(2E,5R)-5-[3-(5-chloropyridin-3-yl)phenyl]-5-cyclopropyl-2-imino-3-methylimidazolidin-4-one 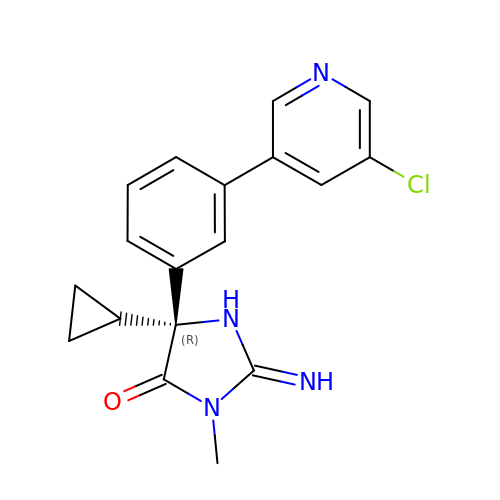| C18 H17 Cl N4 O | SZDQNTKTWBPIBH-GOSISDBHSA-N N-(4-fluorobenzyl)-N-(2-methylpropyl)-6-{[1-(methylsulfonyl)piperidin-4-yl]amino}pyridine-3-sulfonamide | C22 H31 F N4 O4 S2 | 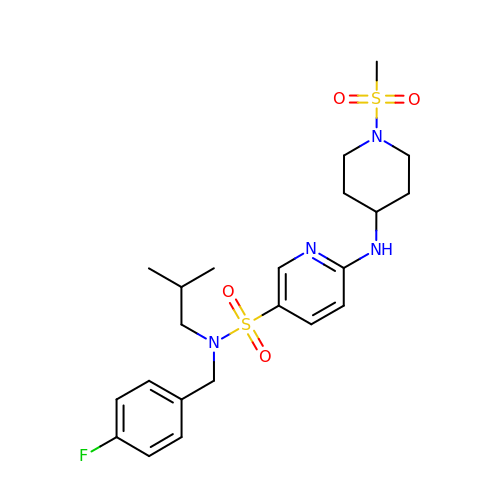AUXZRHVPMQIECB-UHFFFAOYSA-N>[4x]MVQRIYLDNNATTRIDPKVKEIMDPFLRDHYGNPSSLHQFGTETHPAIAEALDKLYKGINARDIDDVIITSCATESNNWVL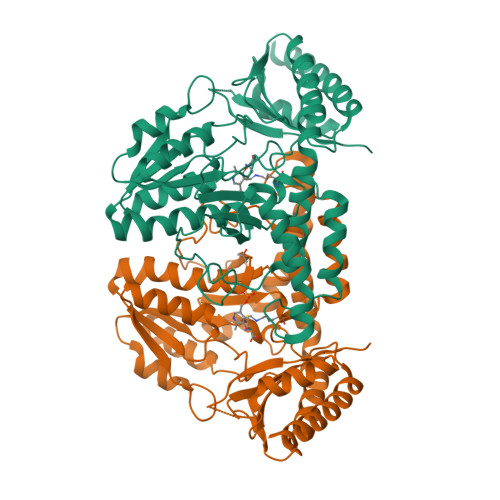KGVYFDECLKKGKNHIVTTVAEHPAVRSTCNFLESLGVEVTYLPINEHGSITAEQVREAITEKTALVSVMWANNETGLIFPIEEIGAICKEKGVLFHTDAVQAIGKIPVDVLKANADFLSFSAHKFHGPKGIGGLYIRSGVGLTPLFHGGEHMNGRRSGTLNVPYIVGMGEAMKLAVEHLDYEKEVVGKLRDKLEEALLKIPDVMVVGDRIHRVPNTTLVSVRGIEGEAMLWDLNRSNIAASTGSACASEDLEANPVMVAIGASKELAHTAIRLSLSRFNTEAEIDKTIEVFSQAAVRLRNISSSYVDLVPRGSHHHHHH ALAREMYCIN 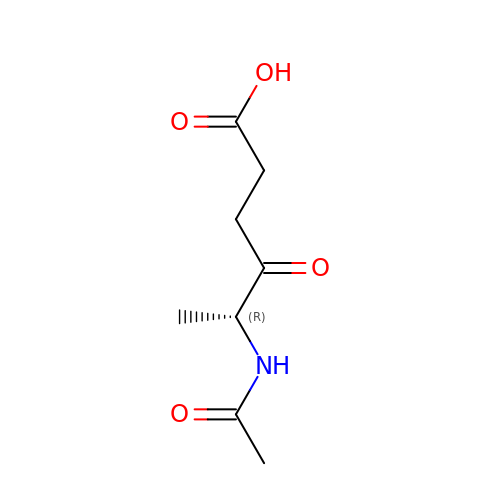2 | C8 H13 N O4 | QSRUAKBTZTXXLM-RXMQYKEDSA-N>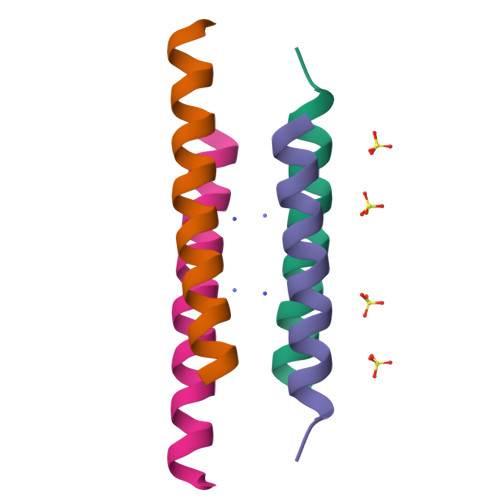[2x]XGELKAIAQELKAIAKELKAIAWEDKAIAQGX>AHMDRIIEKLDHGWWVVSHEQKLWLPKGELPYGEAANFDLVGQRALQIGEWQGEPVWLVQQQRRHDMGSVRQVIDLDVGLF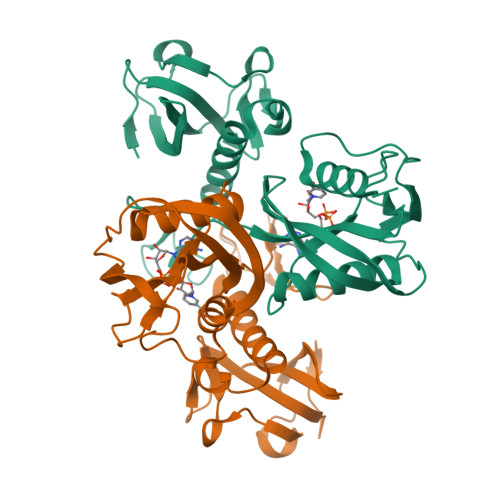QLAGRGVQLAEFYRSHKYCGYCGHEMYPSKTEWAMLCSHCRERYYPQIAPCIIVAIRRDDSILLAQHTRHRNGVHTVLAGFVEVGETLEQAVAREVMEQSGIKVKNLRYVTSQPWPFPQSLMTAFMAEYDSGDIVIDPKELLEANWYRYDDLPLLPPPGTVARRLIEDTVAMCRAEYE[2x]>[8x]AGIVGAIAQRDVAEILLEGLRRLEYRGYDSAGLAVVDAEGHMTRLRRLGKVQMLAQAAEEHPLHGGTGIAHTRWATHGEPSEVNAHPHVSEHIVVVHNGIIENHEPLREELKARGYTFVSETDTEVIAHLVNWELKQGGTLREAVLRAIPQLRGAYGTVIMDSRHPDTLLAARSGSPLVIGLGMGENFIASDQLALLPVTRRFIFLEEGDIAEITRRSVNIFDKTGAEVKRQDIESNLQYDAGDKGIYRHYMQKEIYEQPNAIKNTLTGRISHGQVDLSELGPNADELLSKVEHIQILACGTSYNSGMVSRYWFESLAGIPCDVEIASEFRYRKSAVRRNSLMITLSQSGETADTLAGLRLSKELGYLGSLAICNVPGSSLVRESDLALMTNAGTEIGVASTKAFTTQLTVLLMLVAKLSRLKGLDASIEHDIVHGLQALPSRIEQMLSQDKRIEALA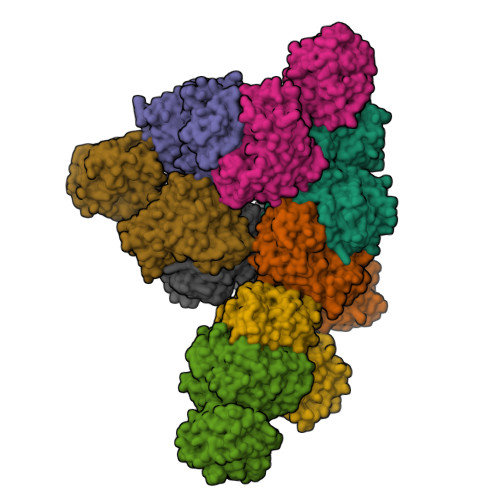EDFSDKHHALFLGRGDQYPIALEGALKLKEISYIHAEAYAAGELKHGPLALIDADMPVIVVAPNNELLEKLKSNIEEVRARGGQLYVFADQDAGFVSSDNMHIIEMPHVEEVIAPIFYTVPLQLLAYHVALIKGTDVDQPRNLAKSVTVE>MSHPDLNKLLELWPHIQEYQDLALKHGINDIFQGNGGKLLQVLL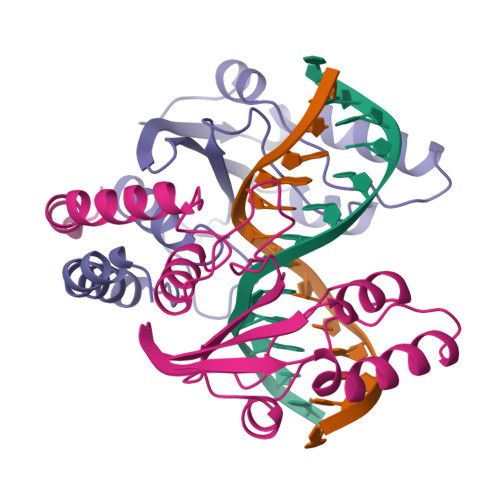ITGLTVLPGREGNDAVDNAGQEYELKSINIDLTKGFSTHHHMNPVIIAKYRQVPWIFAIYRGIAIEAIYRLEPKDLEFYYDKWERKWYSDGHKDINNPKIPVKYVMEHGTKIY[2x]>MALADISGYLDVLDSVRGFSYLENAREVLRSGEARCLGNPRSEPEYVKALYVIGASRIPVGDGCSHTLEELGVFDISVPGEMVFPSPLDFFERGKPTPLVRSRLQLPNGVRVWLKLEWYNPFSLSVKDRPAVEIISRLSRRVEKGSLVADATSSNFGVALSAVARLYGYRARVYLPGAAEEFGKLLPRLLGAQVIVDPEAPSTVHLLPRVMKDSKNEGFVHVNQFYNDANFEAHMRGTAREIFVQSRRGGLALRGVAGSLGTSGHMSAAAFYLQSVDPSIRAVLVQPAQGDSIPGIRRVETGMLWINMLDISYTLAEVTLEEAMEAVVEVARSDGLVIG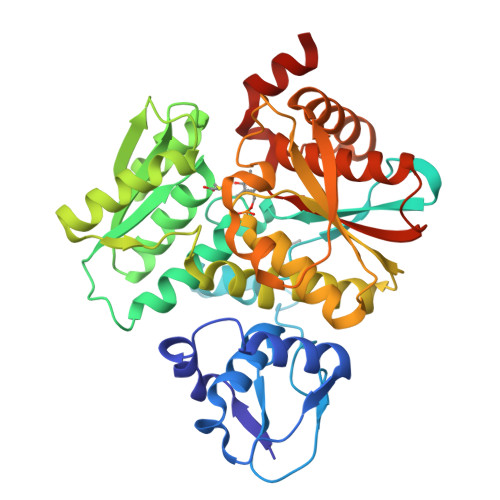PSGGAAVKALAKKAAEGDLEPGDYVVVVPDTGFKYLSLVQNALEGAGDSV[2x]>[2x]SNAMMEVCPY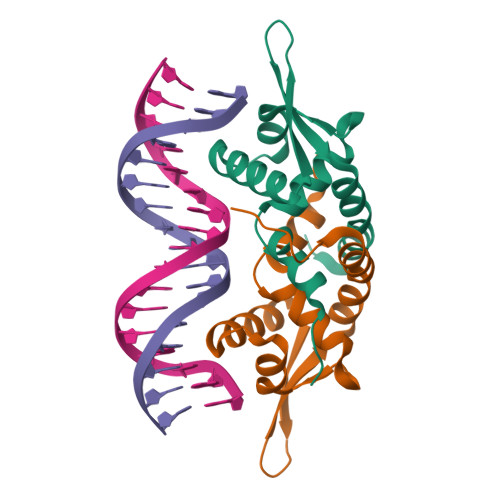LEETFKILGRSWNGLIINYLSRCNDCSAHFSDMKRDLKTITPRALSLKLSELAQWELVEKQIISTSPVQIIYVLTEKGKALAEALHPIEAWAQSYVDLTDQRTAK>MATLTAKNLAKAYKGRRVVEDVSLTVNSGEIVGLLGPNGAGKTTTFYMVVGIVPRDAGNIIIDDDDISLLPLHARARRGIGYLPQEASIFRRLSVYDNLMAVLQIRDDLSAEQREDRANELMEEFHIEHLRDSMGQSLSGGERRRVEIARALAANPKFILLDEPFAGVDPISVIDIKRIIEHLRDSGLGVLITDHNVRETLAVCERAYIV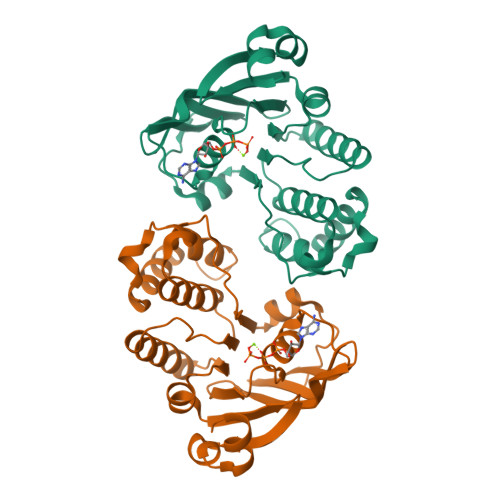SQGHLIAHGTPTEILQDEHVKRVYLGEDFRLHHHHHH[2x]>EHVTGKWFSVPELRLRDHRFIVPLDYSKSSPKITVFAREIVAVGKEEQAMPYLLYLQGGPGFEGPRPSEASGWIQRACEEFRVVLLDQRGTGLSTPLICSSMLQFKSAKELADYLVHFRADNIVKDAEFIRVRLVPKADPWTILGQSFGGFCALTYLSFAPEGLKQVLITGGIPPIGKACTADDVYEAGFEQVARQNEKYYKRFPQDIEIVRELVNYLAESEGGGVPLPSGGILTPKGLQTLGLSGLGSSTGFERLHYMLERVWDPILVTG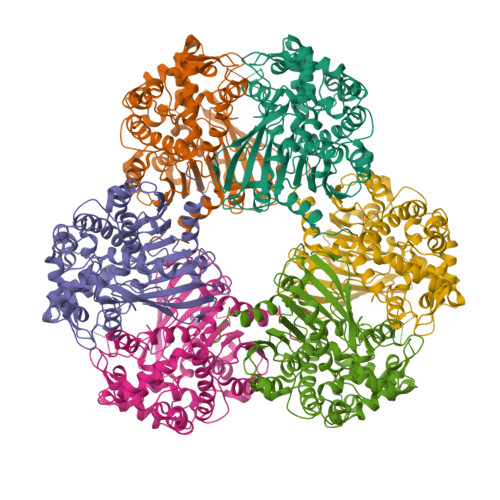APKCISQFFLNAFESWHSFDANPLYALLHEAIYCEGASSGWSAHRLRDKYEYKFDAMKAVKESQPVLFTGEMIFPWMFDEIHALKPFKAAADLLAKKEDWPPLYDVPRLQNNKVPVAAAVYYEDMYVNFKLVTETASHISGIRLWVTNEFMHSGLRDAGRQIIDHLLGMINGKKPLF[6x]N2-(2-Methoxy-4-(1-methyl-1H-pyrazol-4-yl)phenyl)-N8-neopentylpyrido[3,4-d]pyrimidine-2,8-diamine | C23 H27 N7 O | 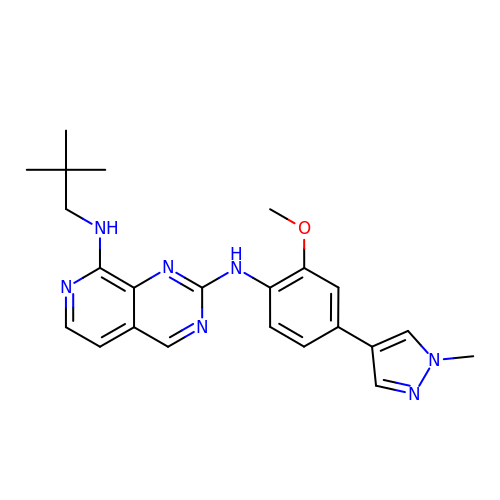WSTCEYSBWKYEDE-UHFFFAOYSA-N> MAHHHHHHVDDDDKENLYFQSKPNLSAKDLALLLFTHLPGNNTPFHILAQVLSKIAYKSGKSGAFLDAFHQILSEGENAQAALTRLSRTFDAFLGVVPPVIRVKNFQTVPRPCQKSLRAVPPNPTIDKGWVCVYSSEQGETRALKI

Filoviruses encode a viral protein termed VP35 which is important for nucleocapsid assembly, replication and transcription and also plays a critical role in host immunosuppression. VP35 binds to and likely masks viral dsRNA from host factors, which leads to suppression of RNA silencing, inhibition of phosphorylation/activation of interferon regulatory factor 3 (IRF-3) and antagonism of the type I IFN response. Here we present the crystal structure of the dsRNA-binding domain (RBD) of Marburg virus VP35, alone and in complex with dsRNA. The structures and accompanying dsRNA-binding analysis performed by dot-blot assays and isothermal titration calorimetry reveal that MARV VP35 RBD coats the sugar-phosphate backbone along the length of dsRNA in addition to capping at the terminus, suggesting an alternate mechanism of dsRNA masking for immunosuppression.

MARV VP35 RBD was crystallized in space group C2221 with one molecule of the VP35 RBD in the asymmetric unit. Interpretable electron density was observed for residues 208–329 of the RBD. Like the VP35 RBDs of EBOV and RESTV, the RBD of MARV VP35 contains α-helical and β-sheet subdomains connected by a short loop. The β-sheet subdomain is formed by a three-stranded mixed β-sheet and an α-helix, and features the conserved, central basic patch critical to dsRNA binding, that contains residues R271, R294, K298, R301, K311, R325 and K328. The α-helical subdomain contains a four-helix bundle followed by a short fifth helix and features the conserved first basic patch containing residues K211, K237 and K241. The RBD of MARV VP35 is 43% and 41% identical in sequence to those of EBOV and RESTV, respectively, and the crystal structures align with a root mean square deviation (r.m.s.d.) of 1.07 Å and 0.92 Å, to EBOV and RESTV respectively. The location and in general, the contents of both the central and first basic patches are conserved among the structures. The residue F228 is located in a hydrophobic pocket that bridges the α-helical subdomain to the β-sheet subdomain.>MRGSHHHHHHGSMVLGKPQTDPTLEWFLSHCHIHKYPSKSTLIHQGEKAETLYYIVKGSVAVLIKDEEGKEMILSYLNQGDFIGELGLFEEGQERSAWVRAKTACEVAEISYKKFRQLIQVNPDILMRLSAQMARRLQVTSEKAGNLAFLDVTGRIAQTLLNLAKQPDAMTHPDGMQIKITRQEIGQIVGCSRETVGRILKMLEDQNLISAHGKTIVVYGTR[2x]

CAP is a 210-amino-acid transcription factor that binds cAMP generated by adenylyl cyclase in response to the phosphorylated form of Enzyme IIAGlc (phosphorylated in response to the phosphoenolpyruvate-carbohydrate phosphotransferase system). cAMP-bound CAP regulates the transcription of over 100 genes crucial for carbon utilization through its binding to a specific promoter region and recruitment of RNA polymerase. Previous studies of the ligand binding domain of CAP demonstrated negative cooperativity between cAMP binding sites in the absence of structural change within this domain. We produce coarse-grained models that describe global low-frequency protein backbone motions of CAP and show a strong correlation between negative cooperativity for cAMP and modulation of the delocalised normal modes on ligand binding without a requirement for a spatially distinct physical pathway or conformational change. We demonstrate experimentally that altered connectivity between backbone elements in CAP can give predictable alterations to cooperativity for cAMP binding through altered mode amplitudes.

We examined amino acids predicted to show altered (V132, H160) or neutral (V140) responses to altered amino acid side chain interactions. The removal (V132A) or addition (V132L) of a side chain methyl group of V132 was engineered to decrease and increase, respectively, the strength of hydrophobic interaction across the dimer interface. Computation predicted that these mutations would result in more negative and positive cooperativity in CAP, respectively and that the most important contacts contributing to this effect were with L62 and V132 of the opposing monomer. High-resolution X-ray crystal structures of CAP mutants V132A and V132L demonstrated that these variants possessed decreased and increased hydrophobic interactions across the dimer interface, respectively. Comparison of variant crystal structures with wild-type demonstrated that there was no statistically significant change in structure. Cooperativity for cAMP binding was studied by isothermal titration calorimetry (ITC) for wild-type, V132A, and V132L proteins to examine whether the experimentally observed changes in cooperativity matched computational predictions.>MDAFQGILKFFLNQKTVIGYSFMALLTVGSERLFSVVAFKCPCSTENMTYGLVFLFAPAWVLLILGFFLNNRSWRLFTGCCVNPRKIFPRGHSCRFFYVLGQITLSSLVAPVMWLSVALLNGTFYECAMSGTRSSGLLELICKGKPKECWEELHKVSCGKTSMLPTVNEELKLSLQAQSQILGWCLICSASFFSLLTTCYARCRSKVSYLQLSFWKTYAQKEKEQLENTFLDYANKLSERNLKCFFENKRPDPFPMPTFAAWEAASELHSFHQSQQHYSTLHRVVDNG[11x]

To further investigate the CALHM channels, we purified human CALHM5 and determined its structure by cryo-electron microscopy (cryo-EM). CALHM5 assembles as an undecamer, showing an overall truncated cone-shaped architecture, with approximate dimensions of 95 Å in height spanning the cell membrane, 125 Å in extracellular width, and 145 Å in intracellular width. Each subunit consists of a large transmembrane domain (TMD) that comprises four transmembrane helices TM1–4 and an N-terminal helix (NTH), an intracellular C-terminal domain (CTD) consisting of three α-helices CH1–3 and an extracellular loop region. CALHM5 exhibits an unusually large pore along the symmetric axis which is broad at both entrances with a measured diameter of ~60 Å and is slightly narrowed down at constriction.

We determined the structures of CALHM5 in the presence of EDTA, Ca2+ or rubidium red (RUR) at overall resolutions of 2.89 Å, 2.90 Å, and 2.64 Å, respectively. However, these regions are well defined in the CALHM5 structure, where TM1 is poised parallel to the central axis of symmetry and the preceding NTH projects toward the axis forming a constriction. We observed extra amorphous density in the middle of the CALHM5 channel and five lipid-like densities per CALHM5 monomer annotated as PA1–5. PA1 is oriented upwards, with headgroups toward positively charged residues at the short extracellular loop. PA2–5 are oriented in the opposite direction within a cavity formed by intracellular halves of TM2–4, where a network of hydrogen bonds and salt bridges holds these lipid phosphates in place. But in our investigated structure of CALHM5, PA1’s hydrophilic head forms hydrogen bonds with surrounding residues including Arg32 of TM1, Asn121 of TM3, and Val37 of TM1′ (apostrophe indicates the adjacent subunit), whereas the hydrophobic tails fill the gap between two adjacent TM1 helices. Interestingly, we noticed that these residues are not conserved among CALHMs and some of them, such as Asn121 and Arg32 (Arg124 and Glu37 in CALHM2), are also involved in RUR binding in CALHM2.> MSAIKPDMKIKLRMEGNVNGHHFVIDGDGTGKPFEGKQSMDLEVKEGGPLPFAFDILTTAFAYGNRVFAKYPDNIQDYFKQSFPKGYSWERSLTFEDGGICNARNDITMEGDTFYN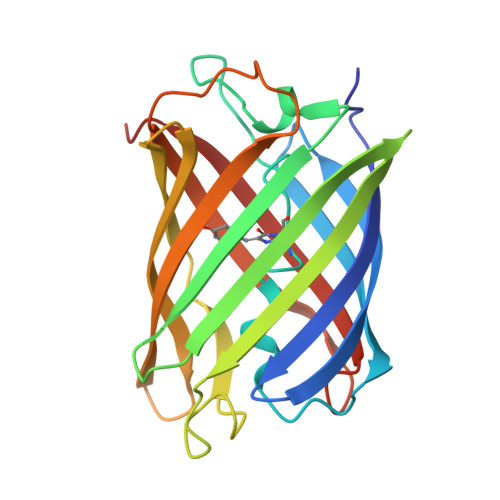KVRFYGTNFPANGPVMQKKTLKWEPSTEKMYVRDGVLTGDVETALLLEGNAHYRCDFRTTYKAKEKGVKLPGAHFVDHCIEILSHDKDYNKVKLYEHAVAHSGLPN>MSPYLVPDTQALCHHLPVIRQLATSGRFIVIIPRTVIDGLDLLKKEHPGARDGIRYLEAEFKKGNRYIRCQKEVGKSFERHKLKRQDADAWTLYKILDSCKQLTLAQGAGEEDPSGMVTIITGLPLDNPSVLSGPMQAA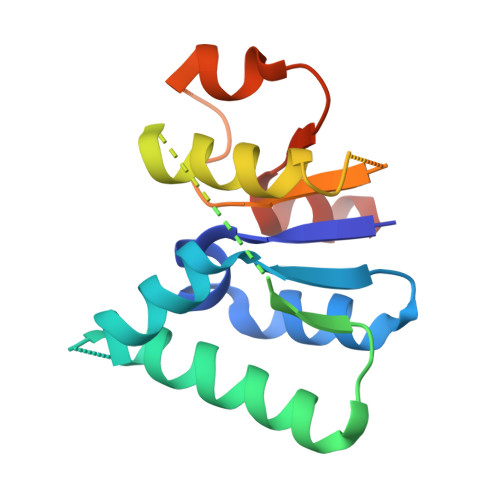LQAAAHASVDIKNVLDFYKQWKEIG[2x]> TGS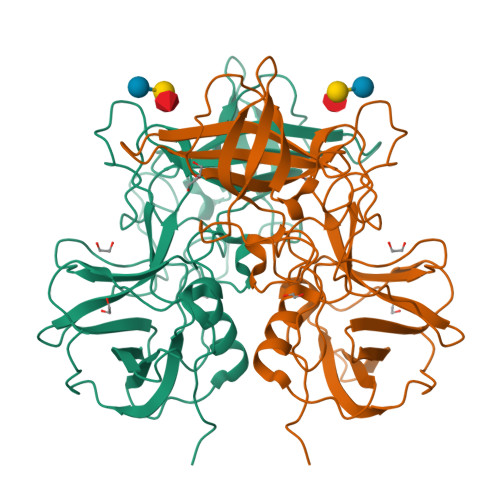KPFSVPVLTVEEMTNSRFPIPLEKLFTGPSSAFVVQPQNGRCTTDGVLLGTTQLSPVNICTFRGDVTHITGSRNYTMNLASQNWNDYDPTEEIPAPLGTPDFVGKIQGVLTQTTRTDGSTRGHKATVYTGSADFAPKLGRVQFETDTDRDFEANQNTKFTPVGVIQDGGTTHRNEPQQWVLPSYSGRNTHNVHLAPAVAPTFPGEQLLFFRSTMPGCSGYPNMDLDCLLPQEWVQYFYQEAAPAQSDVALLRFVNPDTGRVLFECKLHKSGYVTVAHTGQHDLVIPPNGYFRFDSWVNQFYTLAPM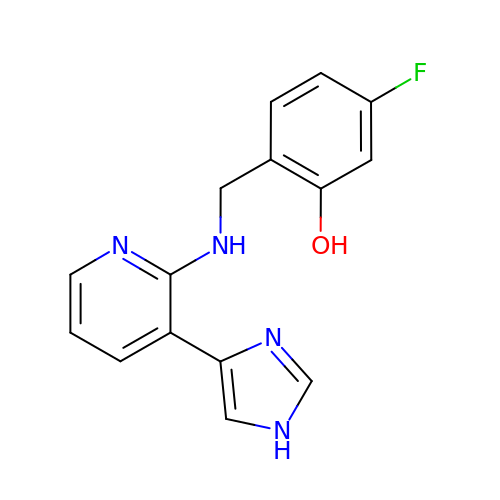5-fluoro-2-({[(3M)-3-(1H-imidazol-4-yl)pyridin-2-yl]amino}methyl)phenol | C15 H13 F N4 O | GOBKDOPCDPTXFF-UHFFFAOYSA-N> MINAIRTPDQRFSNLDQYPFSPNYLDDLPGYPGLRAHYLDEGNSDAEDVFLCLHGEPTWSYLYRKMIPVFAESGARVIAPDFFGFGKSDKPVDEEDYTFEFHRNFL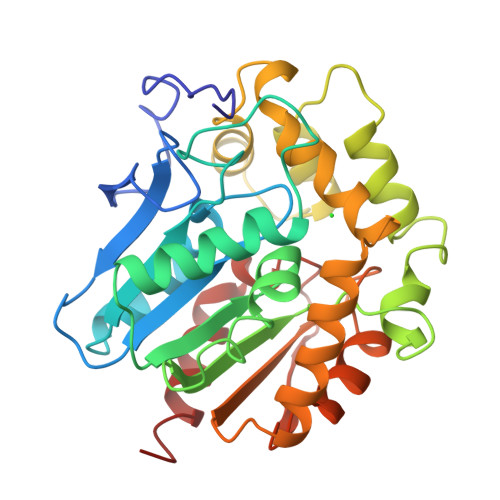LALIERLDLRNITLVVQDWGGFLGLTLPMADPSRFKRLIIMNACLMTDPVTQPAFSAFVTQPADGFTAWKYDLVTPSDLRLDQFMKRWAPTLTEAEASAYAAPFPDTSYQAGVRKFPKMVAQRDQACIDISTEAISFWQNDWNGQTFMAIGMKDKLLGPDVMYPMKALINGCPEPLEIADAGHFVQEFGEQVAREALKHFAETE>GMAEFDAVTAFADAPAAVLSTLNADGAPHLVPVVFAVHVPHVEGQPARIYTAVDAKRKTTRNLRRLANIDRD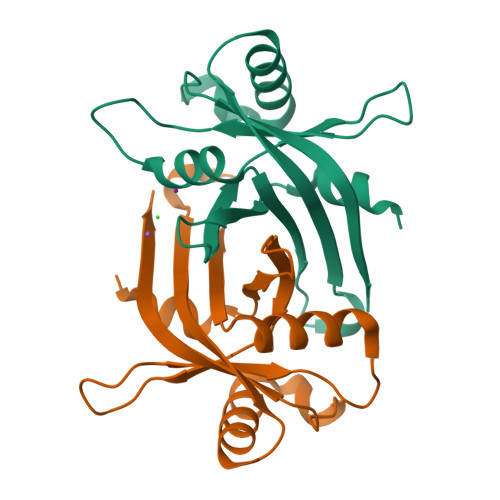SRVSLLVDHYSDDWTQLWWVRADGVATTHHSGDEVATGYALLRAKYHQYERVSLDGPVISVEVSRWASWQA[2x]> XXXXXXXXXXXXXXXXXXXXXXXXXTYLSWEVSVSLSVGFKTMDFPAVTICNASPFKYSKIKHLLKDLDELMEAVLERILAPELSHANATRNLNFSIWNHTPLVLIDERNPHHPMVLDLFGDNHNGLTSSSASEKICNAHGCKMAMRLCSLNRTQCTFRNFTSATQALTEWYILQATNIFAQVPQQELVEMSYPGEQMILACLFGAEPCNYRNFTSIFYPHYGNCYIFNWGMTEKALPSANPGTEFGLKLILDIGQEDYVPFLASTAGVRLMLHEQRSYPFIRDEGIYAMSGTETSIGVLVDKLQRMGEPYSPCTVNGSEVPVQNFYSDYNTTYSIQACLRSCFQDHMIRNCNCGHYLYPLPRGEKYCNNRDFPDWAHCYSDLQMSVAQRETCIGMCKESCNDTQYKMTISMADWPSEASEDWIFHVLSQERDQSTNITLSRKGIVKLNIYFQEFNYRTIEESAA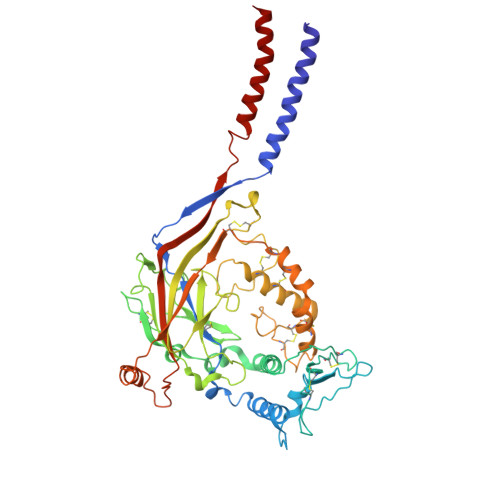NNIXXXXXXXXXXXXXXXXXXXXXXXXXXX>QTPDKAKEQHPKLETYRCTKASGCKKQTNYIVADAGIHGIRQKNGAGCGDWGQKPNATACPDEASCAKNCILSGMDSNAYKNAGITTSGNKLRLQQLINNQLVSPRVYLLEENKKKYEMLHLTGTEFSFDVEMEKLPCGMNGALYLSEMPQDGGKSTSRNSKAGAYYGAGYCDAQCYVTPFINGVGNIKGQGVCCNELDIWEANSRATHIAPHPCSKPGLYGCTGDECGSSGICDKAGCGWNHNRINVTDFYGRGKQYKVDSTRKFTVTSQFVANKQGDLIELHRHYIQDNKVIESAVVNISGPPKINFINDKYCAATGANEYMRLGGTKQMGDAMSRGMVLAMS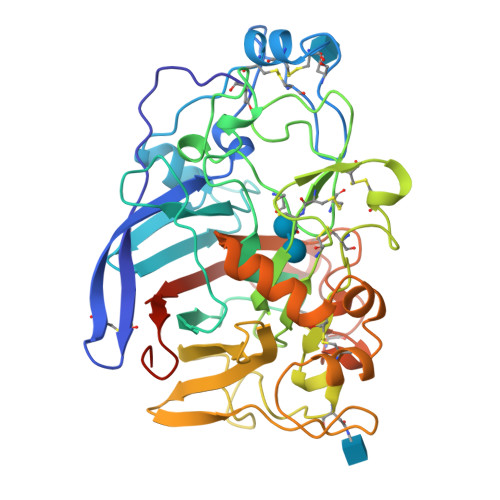VWWSEGDFMAWLDQGVAGPCDATEGDPKNIVKVQPNPEVTFSNIRIGEIGSTSSVKAPAYPGPHRL[4x]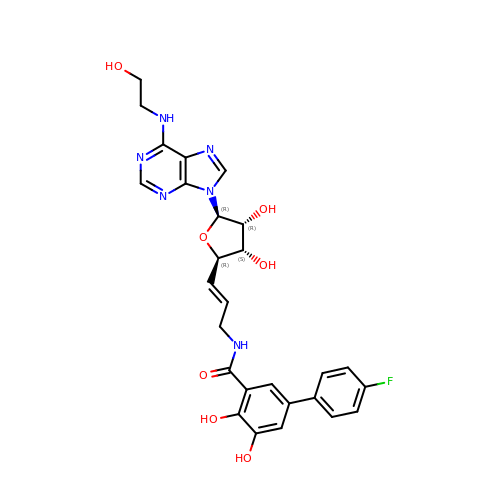N-[(E)-3-[(2R,3S,4R,5R)-3,4-dihydroxy-5-[6-(2-hydroxyethylamino)purin-9-yl]oxolan-2-yl]prop-2-enyl]-5-(4-fluorophenyl)-2,3-dihydroxy-benzamide | C27 H27 F N6 O7 | HBNVZKRROMJMCF-RBUFWCAOSA-N>[2x]DCYCR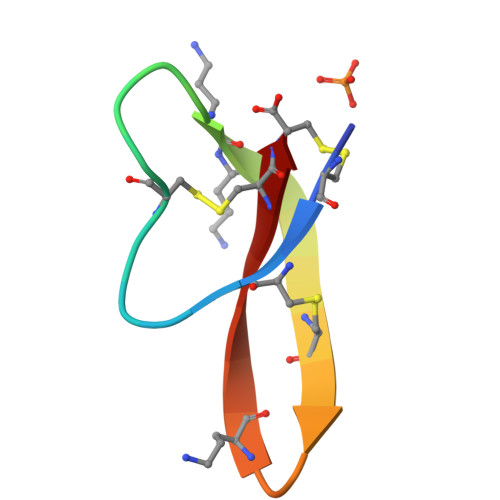IPACIAGEAAYGTCIYQGALWAFCC> GHHHHHHMDDIKVFQNEVLGTLQRGKEENISCDNLVLEINSLKYAYNIS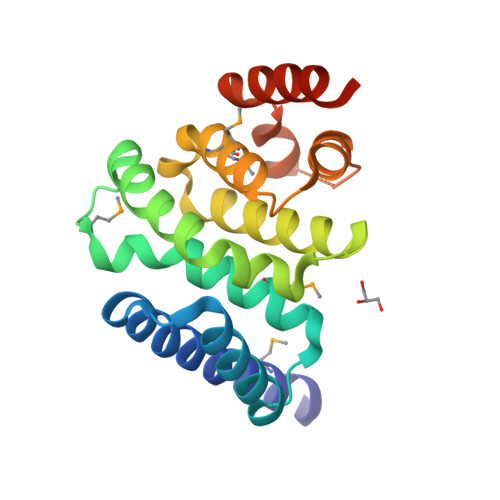LKEVMQVLSHVVLEFPLQQMDSPLDSSRYCALLLPLLKAWSPVFRNYIKRAADHLEALAAIEDFFLEHEALGISMAKVLMAFYQLEILAGETILSWFSQRDTTDKGQQLRKNQQLQRFIQWLKEAEEESSEDD>[2x]SHVDPRIQGELEKLNQSTDDINRRETELEDARQKFRSVLVEATVKLDELVKKIGKAVEDSKPYWEARRVARQAQLEAQKATQDFQRATEVLRAAKETISLAEQRLLEDDKRQFDSAWQEMLNHATQRVMEAEQTKTRSELVHKETAARYNAAMGRMRQLEKKLKRAINKSKPYFELKAKYYVQLEQLKKTVDDLQAKLTLAKGEYKMALKNLEMISDEIHEAAASSAM

The Rab11 subfamily plays important roles in specific trafficking events such as exocytosis, endosomal recycling, and cytokinesis. SH3BP5 and SH3BP5-like (SH3BP5L) proteins have recently been found to serve as guanine nucleotide exchange factors (GEF) for Rab11. SH3BP5 exhibits a V-shaped structure comprising two coiled coils. The coiled coil composed of α1, and α4 is solely responsible for the Rab11a binding and GEF activity.

Because computational secondary structure prediction assigned the N- and C-terminal regions as mostly disordered regions, we selected the central helical region for crystallography. We found that the R260A/R261A/R262A triple mutation reduced the degradation and obtained diffraction-quality crystals. This construct of SH3BP5 (41–266; R260A/R261A/R262A) is hereafter referred to as SH3BP5-RA. Finally, we determined the crystal structures of SeMet SH3BP5-RA/M167A in two different crystal forms (I41 and P41) and native SH3BP5-RA at 3.35, 3.6, and 3.8 Å resolutions, respectively. The asymmetric units of the I41 and P41 crystals contain one and two SH3BP5 molecules, respectively. Therefore, we obtained five different apo-SH3BP5 structures in total (i.e., one from I41 SeMet SH3BP5-RA/M167A, two from P41 SeMet SH3BP5-RA/M167A, and two from P41 native SH3BP5-RA). Although these five apo-SH3BP5 structures exhibit a similar V-shaped conformation, the superposition of these five apo-SH3BP5 structures using α1 as the reference shows some flexibility of the conformation. The hinge region of the V shape contains staggered hydrophobic interactions so as to maintain the V shape.>[2x]MGKEALLNLYRIEYRPKDTTFTVFKPTHEIQKEKLNKVRWRVFLQTGLPTFRREDEFWCAGKVEKDTLYLTLSNGEIVELKRVGEEEFRGFQNERECQELFRDFLTKTKVKDKFISDFYKKFRDKITVQGKNRKIALIPEVNEK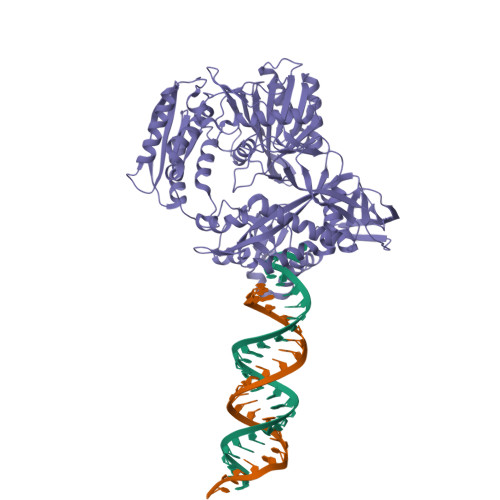VLKSEEGYFLLHLDLKFRIQPFETLQTLLERNDFNPKRIRVKPIGIDFVGRVQDVFKAKEKGEEFFRLCMERSTHKSSKKAWEELLKNRELREKAFLVVLEKGYTYPATILKPVLTYENLEDEERNEVADIVRMEPGKRLNLIRYILRRYVKALRDYGWYISPEEERAKGKLNFKDTVLDAKGKNTKVITNLRKFLELCRPFVKKDVLSVEIISVSVYKKLEWRKEEFLKELINFLKNKGIKLKIKGKSLILAQTREEAKEKLIPVINKIKDVDLVIVFLEEYPKVDPYKSFLLYDFVKRELLKKMIPSQVILNRTLKNENLKFVLLNVAEQVLAKTGNIPYKLKEIEGKVDAFVGIDISRITRDGKTVNAVAFTKIFNSKGELVRYYLTSYPAFGEKLTEKAIGDVFSLLEKLGFKKGSKIVVHRDGRLYRDEVAAFKKYGELYGYSLELLEIIKRNNPRFFSNEKFIKGYFYKLSEDSVILATYNQVYEGTHQPIKVRKVYGELPVEVLCSQILSLTLMNYSSFQPIKLPATVHYSDKITKLMLRGIEPIKKEGDIMYWL> MPKVYNSIVVDAPVERVWSRIRNFHDFSWAPSLIKSC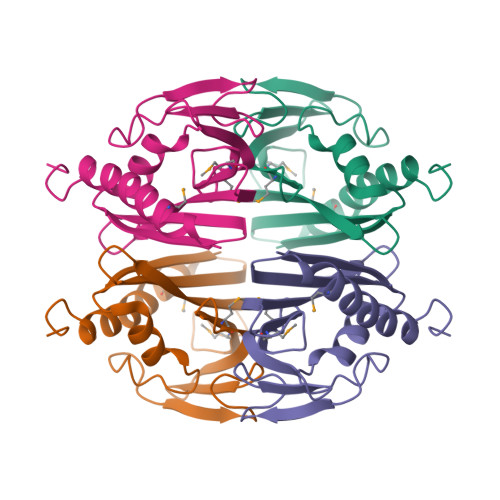KKVGGGGGYSVGARRLLNGEFLDTLIAYSEIERRIMYSMDEGPSPVSSGEIYNYVGNLHLLPVTIDDTTFVEWSGSWESASTEAVEYMNTVYRSLLADLAAEFTSESRRSEWIDQLEHHHHHH>MIYPIFIFKTVEGFDGYFPDIDGCFFAGNTFADISKNAEEAFAVHIEALMNEGFPLPSPPKDPHRYIDDPRLKEEGGILGFVEIDPAKYESKAVKFNLTMSQNLLTAIDKFIATNRGYKNRSQFLAELAREKIISLEHHHHHH[2x];>[2x]MESGELIKRLEDAGW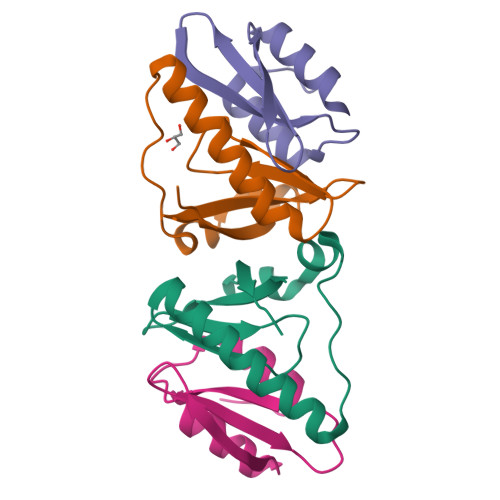QIRGGRKTNSGSHVTLCKPGVRKIITLPYPRKDISKGLLRQAQKIAGIKLS Here, we describe a phage tailspike protein, named K2-2, that specifically depolymerizes the K2 capsular polysaccharide (CPS) of K. pneumoniae into tetrasaccharide repeating units. During the initial stage of infection, the tailspike proteins (TSPs) of bacteriophage recognize specific polysaccharides on the surface of the host cell and attach to them for adsorption. TSPs, also known as polysaccharide depolymerases, have the function of binding and digesting CPS. TSPs typically consist of three domains: an N-terminal particle-binding domain that connects to the tail structure or baseplate of the phage, a receptor-binding domain that extends from the homotrimeric structure and is responsible for host recognition and catalytic activity, and a C-terminal domain that plays a vital role in trimer formation, receptor binding, and intra-molecular chaperone functions.

The sugar-bound crystals were subsequently obtained by soaking the E323A crystals in the crystallization solution added with the hydrolyzed K2 CPS products for 18–24 h. The complex structure was solved at 1.58 Å resolution. Interestingly, the sugar binding changed the space group of the crystals from P21 to C2, resulting in a single trimer of the enzyme in the asymmetric unit. The product-bound structure revealed three equivalent intersubunit carbohydrate-binding grooves in a trimer; two were bound with a dodecasaccharide, while the third had only one tetrasaccharide. Surprisingly, adjacent to the residues Ala323 (mutated from Glu323) and Glu267* that served as a boundary, the bound dodecasaccharide was, indeed, divided into a tetrasaccharide and an octasaccharide, which corresponded to the one and two tetrasaccharide repeating units identified in the hydrolyzed products of K2 CPS. This finding strongly supports Glu267 and Glu323 to be the catalytic residues, which allows for the numbering of the polysaccharide chain from −3 to +6 based on the direction from the non-reducing end to the reducing end. Furthermore, as judged by the clear electron density, we observed an O-acetylation at the C6-OH of +4 Manp. The bound dodecasaccharide lies in an elongated intersubunit groove, with the orientation of its two-repeating-unit chain nearly parallel to the longitudinal axis of the β-helix and the single-repeating-unit perpendicular to the longitudinal axis, reminiscent of the intersubunit carbohydrate-binding site reported for Sf6 TSP and ФAB6 TSP. Notably, the C6-carboxyl group at the branched glucuronic acid that connects to −3 Manp formed a salt bridge with the residue Arg331 and a hydrogen bond to Ser327, suggesting a crucial role of this carboxyl group in the K2 CPS recognition by the enzyme. The distance between Glu323WT and Glu267* is ~4.9 Å, in good agreement with the typical distance between the catalytic nucleophile and general acid/base in a retaining glycosidase, i.e., 4.5–5.5 Å (35).

>MGHHHHHHHHHHSSGHGTIQGSEDLYFQSHMMALVDLVRAGGYSVEYPQFSSMAKLKAFPHSEDGQLVRLLSWHEGVGLGGGLFKVSTSSTATGNDGTVVVASNGVRLLRVVNGPIWADMFGALPNSDIDSMPAVAAAYAYAASVNTDLYIGVATYKFKGSTPINVDPSRAGIIGYQGKVRIDCSEFTGSIVFSINSSYSYTPAAYYNNLSPALQGLYVFGAKTSGVDGLLVGRETVGSDKSYNGQTEVRECTFDKFDRNIRMGHNSWRFVFYKVNSLNALSPNGILYVPAGLDDSGEILSFYHCQFFDGAGSNIRLSCSSYTMVFNTCSFLNITFFVDSASSATVTCNGCNFANPGSASTRRYVDISAGHTNVFNIIGGSIVTNSNPGQTQALLYVSTDNLLNLVGVTAPYGGHYQQEQELGYHAFIGGAGTVTTSGVMLQLRNGAGTCPLHSSLSTFSNWNFGYGNLNAWTVDKGTGTSSVVEYLANAGPKGTEGAMRVAPVSVGTNVSQVQAVTNPGMFSMSCMVNIATTPGNAGQVSIGFLDAAGNSLPGGVSANLGTTTGWQVIGKNTLRGKVPIGAKQVRVNIQTVAGADVKYAYLLCNVVKKLGC[3x]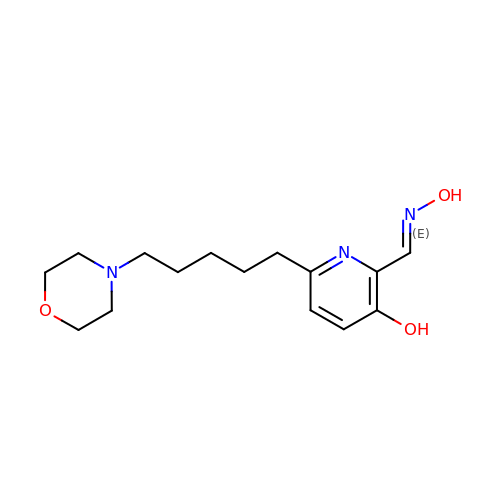2-[(~{E})-hydroxyiminomethyl]-6-(5-morpholin-4-ylpentyl)pyridin-3-ol | C15 H23 N3 O3 | DHXJJCCCAIXLRS-FOWTUZBSSA-N>RDRMVMGKIKRIEAGLPLTTAKGRTFGYDVIDTKLYINEEEAKQLRLIYDIFEEEQSITFLQKRLKKLGFKVRTYNRYNNWLTNDLYCGYVSYKDKVHVKGIHEPIISEEQFYRVQEIFSRMGKNPNMNKESASLLNNLVVCSKCGLGFVHRRKDTVSRGKKYHYRYYSCKTYKHTHELEKCGNKIWRADKLEELIIDRVNNYSFASRNIDKEDELDSLNEKLKIEHAKKKRLFDLYINGSYEVSELDSMMNDIDAQINYYEAQIEANEELKKNKKIQENLADLATVDFNSLEFREKQLYLKSLINKIYIDGEQVTIEWLLEHHHHHH[4x]

The large serine recombinases (LSRs) are DNA-rearranging enzymes that are members of the serine recombinase superfamily. Many LSRs are bacteriophage integrases (often referred to as serine integrases) whose function is to integrate the phage genome into a host chromosome by using short specific DNA sequences, or ‘attachment sites’, in the virus (attP) and in the host (attB). During the integration reaction, LSRs bind to attP and attB as dimers, mediate association of the sites to form a tetrameric synaptic complex and catalyze strand exchange to generate an integrated prophage and new attachment sites, attL and attR. The LSRs share a catalytic domain with the smaller resolvase/invertase enzymes, and there is a strong consensus that the LSRs use the same mechanism of strand exchange.

We crystallized the LI integrase CTD (residues 133–452) bound to a 26-bp A118 attP half-site and determined the structure using anomalous scattering data from selenomethionine-substituted protein and intrinsically bound Zn ions. The integrase CTD is composed of two structural domains: a mixed α/β ‘recombinase domain’ (RD) and a zinc-nucleated domain (ZD) containing an embedded CC motif that extends away from the RD and the DNA. The construct used for crystallization contains part of the helix (αE) that connects the N-terminal catalytic domain (NTD) and RD and is involved in formation of the subunit rotation interface during strand exchange. Together with αE, residues in the integrase CTD make contiguous contact with the entire attP half-site via alternating major and minor groove interactions. The four independent complexes in the asymmetric unit of the crystal are similar everywhere except in the CC motifs, which adopt distinct trajectories. For LI integrase, zinc is coordinated by Cys274 and Cys277, positioned in the β10–β11 turn, and Cys302 and Cys314 positioned in the loop between β12 and αJ. The zinc-coordinating strands form a continuous β-sheet, with β11–β12 engaging the DNA major groove. At the end of the ZD motif, the side chains of Tyr295 and Tyr297 from β12 lie on the surface created by the 5-methyl groups of T24, T23 and T22. From αH, Tyr207 contacts the 5-methyl group of T11, and Asn208 forms a network of hydrogen bonds to the A-T base pairs involving T9 and T10. In addition, the Met136 side chain from αE intercalates between the G0 and T1 bases in all four int–DNA complexes in the asymmetric unit.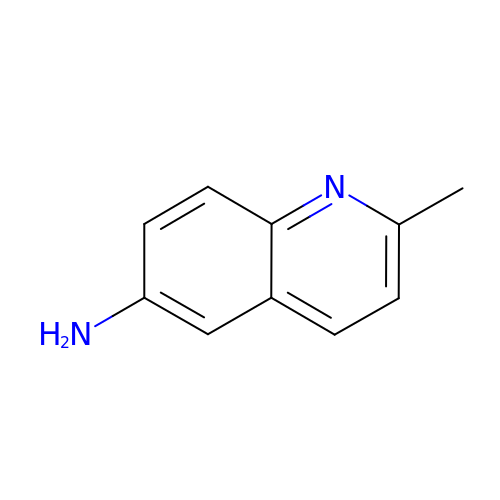2-methylquinolin-6-amine | C10 H10 N2 | TYJFYUVDUUACKX-UHFFFAOYSA-N> GSLKVYNSIFDQAYEIDPIPYFNFLRKHDPVHYEESIDAYFVSKYKDVKYILKNNDIFNTKTLAKRAEPVMKDRVLAQMSGQ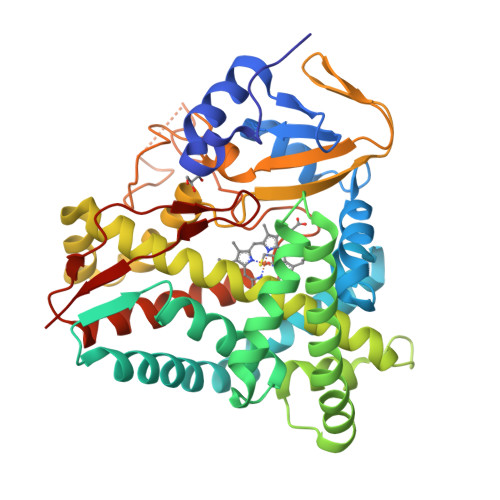EHKSKKKAILKGMTGKYLENLMPILEKRTNDIINKHIEKKEIDIVNDFGKVFAVQSSMDLLGINLENYEKIREWHNGIAKFITSFNLNDEEIKYSLECSDKLENYLMPLIKDRKKSTKDDLISILLEYKNDENSISDTEILALSLNVLLAATEPVDKTLAYLFYNLLKNPEQFESVKNNPKLIKNAIIETLRYNSPVQLIPRQVSKPFIFNNTELQAGDTVICMIGSANRDPEAYSNPDEFNIHRSSDNKSPFTSHSQNLSFGTGVHTCVGASFSLIQLEMVAILLLKRLKNIKLKTMEITEHGIYTRGPKSMVISFD>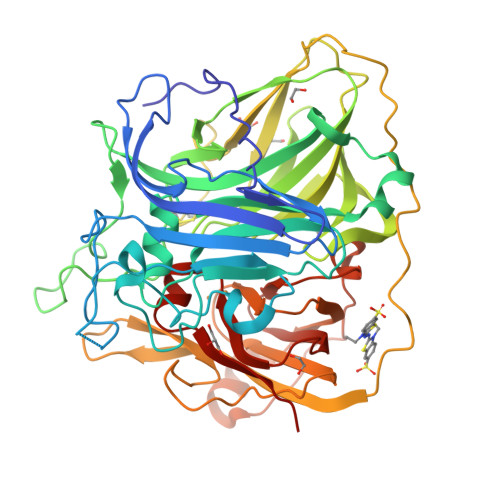 MTLEKFVDALPIPDTLKPVQQSKEKTYYEVTMEECTHQLHRDLPPTRLWGYNGLFPGPTIEVKRNENVYVKWMNNLPSTHFLPIDHTIHHSDSQHEEPEVKTVVHLHGGVTPDDSDGYPEAWFSKDFEQTGPYFKREVYHYPNQQRGAILWYHDHAMALTRLNVYAGLVGAYIIHDPKEKRLKLPSDEYDVPLLITDRTINEDGSLFYPSAPENPSPSLPNPSIVPAFCGETILVNGKVWPYLEVEPRKYRFRVINASNTRTYNLSLDNGGDFIQIGSDGGLLPRSVKLNSFSLAPAERYDIIIDFTAYEGESIILANSAGCGGDVNPETDANIMQFRVTKPLAQKDESRKPKYLASYPSVQHERIQNIRTLKLAGTQDEYGRPVLLLNNKRWHDPVTETPKVGTTEIWSIINPTRGTHPIHLHLVSFRVLDRRPFDIARYQESGELSYTGPAVPPPPSEKGWKDTIQAHAGEVLRIAATFGPYSGRYVWHCHILEHEDYDMMRPMDITDPHK BlaR1 and MecR1 are membrane proteins with an N-terminal zinc metalloprotease domain and a C-terminal extracellular β-lactam-binding sensor domain. β-Lactam binding to the extracellular BlaR1 sensor domain regulates BlaI cleavage by the zinc metalloprotease domain in the cytoplasm. BlaR1 forms a domain-swapped dimer, with the zinc metalloprotease active site accessible from the cytoplasm. BlaR1 undergoes spontaneous autocleavage in cis between Ser283 and Phe284 and we describe the catalytic mechanism and specificity underlying the self and BlaI cleavage.

As in S. aureus and E. coli, BlaR1(WT) expressed in L. lactis undergoes spontaneous autocleavage between residues Ser283 and Phe284 (confirmed by Edman N-terminal sequencing), which was mitigated by mutation of Phe284 in the P1′ position to alanine (BlaR1(F284A)). The structures of BlaR1(WT) and BlaR1(F284A) (the latter alone and in complex with ampicillin) were determined using cryo-electron microscopy (cryo-EM) to nominal resolutions of 3.8–4.6 Å. The BlaR1(F284A) structure (refined with C2 symmetry) exhibited less variability and the sensor domains adopt a position slightly closer to the membrane compared with BlaR1(WT). In the BlaR1(WT) dataset, the sensor domains were observed to be dynamic and are able to adopt different orientations with respect to each other and the transmembrane domains. A comparison with BlaR1(F284A) shows that the sensor domains are positioned at different distances to the transmembrane domain in order of BlaR1(WT), BlaR1(F284A) and BlaR1(F284A)–ampicillin. In the BlaR1(F284A) mutant structures, the autocleavage loop is intact; however, in the BlaR1(WT) structure, we detected a mixture of uncleaved and cleaved forms, the latter with the central P1′ Phe284 slightly shifted in position. Although we observed the same binding orientation in the autocleavage-deficient BlaR1(F284A) structure, the P1′ alanine mutant leads to the loss of the close van der Waals-driven socketing of the aromatic phenylalanine side chain into the S1′ pocket, preventing productive coordination of the carbonyl oxygen to the zinc. The F284A mutation results in an unoccupied S1′ pocket and associated movement of Tyr261 on helix α8 towards His201 of the HEXXH motif in b (orange) and c (cyan; dashed line). The strain containing BlaR1(F284A) (blaR1(F284A)-blaI) displayed intermediate growth attenuation in presence of nafcillin compared with either wild-type BlaR1 (blaR1-blaI) or the functionally defective BlaR1 (null) (blaR1(null)-blaI), showing that the F284A mutant is partially functional.

>MAKLLIMSIVSFCFIFLLLLFFRYILKRYFNYMLNYKVWYLTLLAGLIPFIPIKFSLFKFNNVNNQAPTVESKSHDLNHNINTTKPIQEFATDIHKFNWDSIDNICTVIWIVLVIILSFKFLKALLYLKYLKKQSLYLNENEKNKIDTILFNHQYKKNIVIRKAETIQSPITFWYGKYIILIPSSYFKSVIDKRLKYIILHEYAHAKNRDTLHLIIFNIFSIIMSYNPLVHIVKRKIIHDNEVEADRFVLNNINKNEFKTYAESIMDSVLNVPFFNKNILSHSANGKKSLLKRRLINIKEANLKKQSKLILIFICIFTFLLMVIQSQFLMGQSITDYNYKKPLHNDYQILDKSKIFGSNSGSFVMYSMKKDKYYIYNEKESRKRYSPNSTYKIYLAMFGLDRHIINDENSRMSWNHKHYPFDAWNKEQDLNTAMQNSVNWYFERISDQIPKNYTATQLKQLNYGNKNLGSYKSYWMEDSLKISNLEQVIVFKNMMEQNNHFSKKAKNQLSSSLLIKKNEKYELYGKTGTGIVNGKYNNGWFVGYVITNHDKYYFATHLSDGKPSGKNAELISEKILKEMGVLNGQELALVPRGSSAHHHHHH[2x]> MRVTMSLEALTTEALAAIAAAQDLVALDQVRVQFTGKKSQLAEQSKALGKMDPEERKVQGAAIHAVRETINNALTERQTALQQAALAQKLASETIDITLPGRGQRIGTVHPVTQVQERICQFFTKAGFTVATGPEVEDDYHNFEALNIPGHHPARAMHDTFYFDANHLLRTHTSGVQIRTMETSQPPIRIVCPGRVYRCDSDQTHSPMFHQIEGLYVAENTSFAELKGLLINLLNEFFEKDLKVRFRPSYFPFTEPSAEVDIMDERGRWLEVLGCGMVHPNVLRAAGIDPDKYKGFAFGLGVERFAMLRYGINDL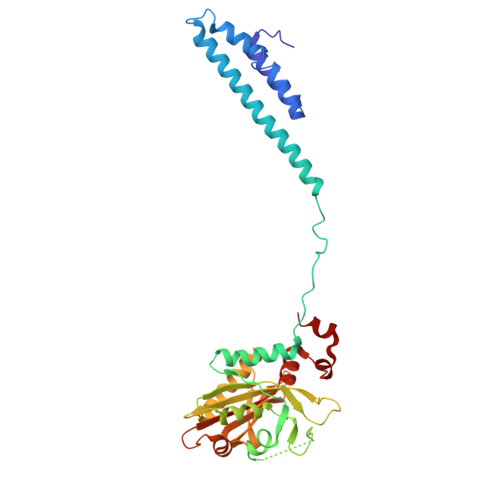RMFYQNDVRFLRQFA> HMPRVKLGTQGLEVSKLGFGCMGLSGDYNDALPEEQGIAVIKEAFNCGITFFDTSDIYGENGSNEELLGKALKQLPREKIQVGTKFGIHEIGFSGVKAKGTPDYVRSCCEASLKRLDVDYIDLFYIHRIDTTVPIEITMGELKKLVEEGKIKYVGLSEASPDTIRRAHAVHPVTALQIE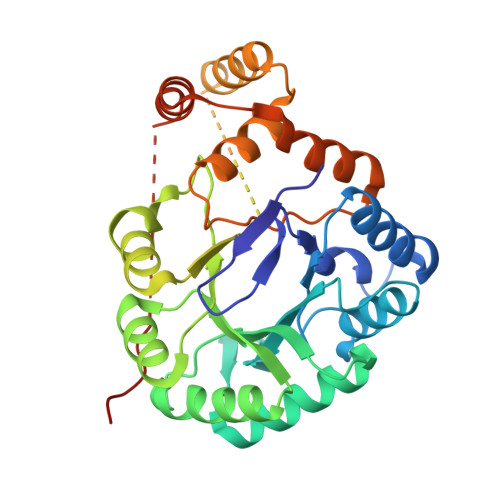YSLWTRDIEDEIVPLCRQLGIGIVPYSPIGRGLFWGKAIKESLPENSVLTSHPRFVGENLEKNKQIYYRIEALSQKHGCTPVQLALAWVLHQGEDVVPIPGTTKIKNLHNNVGALKVKLTKEDLKEISDAVPLDEVAGESIHEVIAVTNWKFANTPPLK>[4x]MGSSHHHHHHSSGLVPRGSHSWQSSSEQKSLAERYLQQIAQSEALRIQQELNYARDVAHNLGQGLAALPSAGIKDRAVVDKMMEYALRDNPEYLSISVIFEENVFDGRDAEFADQPGQAPKGRYA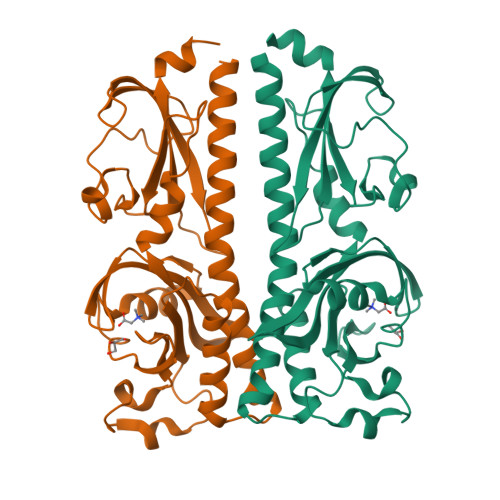WFVDRDQAGNYAMHPLLSYLTPGQGDYYLLPQKSQKDTLIEPYTYAYNGVPTLLTSVAAPIVSQGKLWGVVTSDISLASLQQKINQIKPWEGGGYAMLLSSAGKVISYPDKSQTSKAWQGPTDNFTSSVVQHDDAILGEQALVTWQPVTIGNSTEKWYLGIVVPVSQVMAASERQL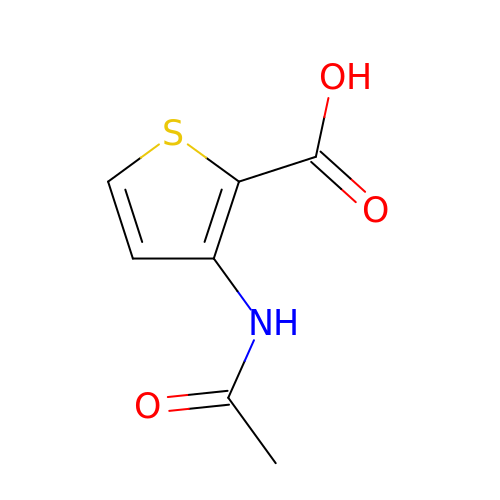3-(acetylamino)thiophene-2-carboxylic acid | C7 H7 N O3 S | LLKLTQJOEPWBOE-UHFFFAOYSA-N> MCHQQLVISWFSLVFLASPLVAIWELKKDVYVVELDWYPDAPGEMVVLTCDTPEEDGITWTLDQSSEVLGSGKTLTIQVKEFGDAGQYTCHKGGEVLSHSLLLLHKKEDGIWSTDILKDQKEPKNKTFLRCEAKNYSGRFTCWWLTTISTDLTFSVKSSRGSSDPQGVTCGAATLSAERVRGDNKEYEYSVECQEDSACPAAEESLPIEVM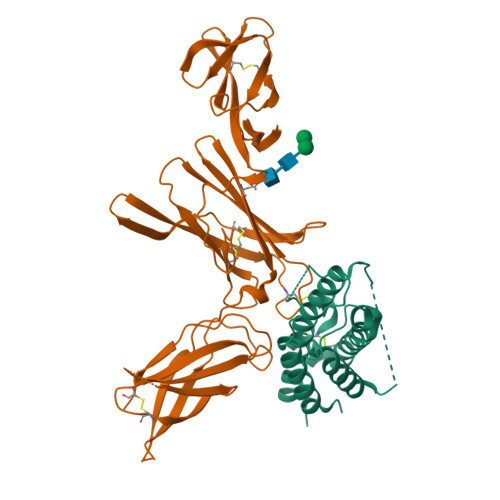VDAVHKLKYENYTSSFFIRDIIKPDPPKNLQLKPLKNSRQVEVSWEYPDTWSTPHSYFSLTFCVQVQGKSKREKKDRVFTDKTSATVICRKNASISVRAQDRYYSSSWSEWASVPCS;> MLGSRAVMLLLLLPWTAQGRAVPGGSSPAWTQCQQLSQKLCTLAWSAHPLVGHMDLREEGDEETTNDVPHIQCGDGCDPQGLRDNSQFCLQRIHQGLIFYEKLLGSDIFTGEPSLLPDSPVGQLHASLLGLSQLLQPEGHHWETQQIPSLSPSQPWQRLLLRFKILRSLQAFVAVAARVFAHGAATLSPGTKHHHHHH2-[(3,5-dimethyl-1,2-oxazol-4-yl)methoxy]-~{N}-(2-methoxyphenyl)benzamide 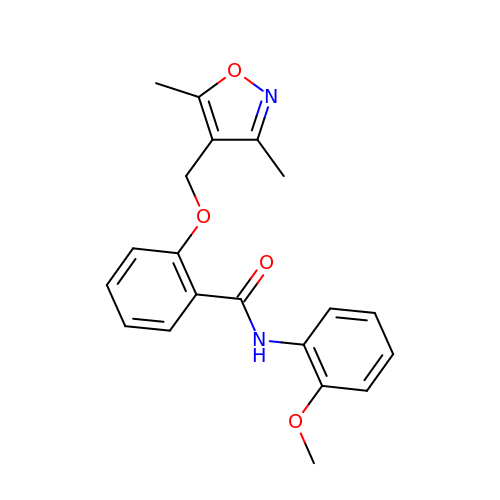| C20 H20 N2 O4 | JUPXIAWRJFYWOF-UHFFFAOYSA-N> MPQISRQEYAGLFGPTTGDKIRLGDTNLFIEIEKDLRGYGEESVYGGGKSLRDGMGANNHLTRDNGVLDLVITNVTIVDARLGVIKADVGIRDGKIAGIGKSGNPGVMDGVTPGLVVGVSTDAISGEHLILTAAGIDTHIHLISPQQAYHALSNGVATFFGGGIGPTDGTNGTTVTPGPWNIRQMLRSVEGLPVNVGILGKGNSYGRGPLLEQAIAGVVGYKVHEDWGATANALRHSLRMADEMDIQVSVHTDSLNECGYVEDTIDAFEGRTIHTFHTEGAGGGHAPDIIRVASQPNVLPSSTNPTLPYGVNSQAELFDMIMVCHNLNPNVPADVSFAESRVR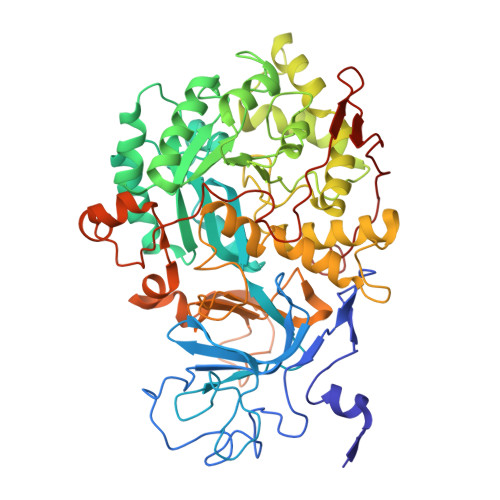PETIAAENVLHDMGVISMFSSDSQAMGRVGENWLRVMQTANAMKASRGKLPEDAPGNDNFRVLRYVAKITINPAIAQGVSHVIGSVEVGKMADLVLWDPRFFGAKPKMVIKGGMINWAAMGDPNASLPTPQPVFYRPMFGAMGKTMQDTCVTFVSQAALDDGVKEKAGLDRQVIAVKNCRTISKHDLVRNDQTPNIEVDPETFAVKVDGVHATCEPIDTAAMNQRYFFG> ALEEAPWPPPEGAFVGFVLSRKEPMWADLLALAAARGGRVHRAPEPYKALRDLKEARGLLAKDLSVLALREGLGLPPGDDPMLLAYLLDPSNTTPEGVARRYGGEWTEEAGERAALSERLFANLWGRLEGEERLLWLYREVERPLSAVLAHMEATGVRLDVAYLRALSLEVAEEIARLEAEVFRLAGHPFNLNSRDQ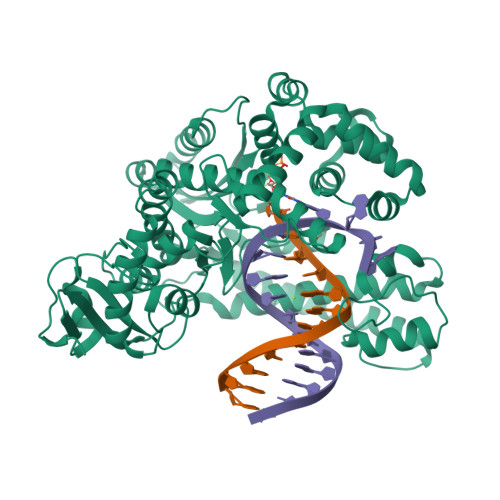LERVLFDELGLPAIGKTEKTGKRSTSAAVLEALREAHPIVEKILQYRELTKLKSTYIDPLPDLIHPRTGRLHTRFNQTATATGRLSSSDPNLQNIPVRTPLGQRIRRAFIAEEGWLLVALDYSQIELRVLAHLSGDENLIRVFQEGRDIHTETASWMFGVPREAVDPLMRRAAKTINFGVLYGMSAHRLSQELAIPYEEAQAFIERYFQSFPKVRAWIEKTLEEGRRRGYVETLFGRRRYVPDLEARVKSVREAAERKAFNMPVQGTAADLMKLAMVKLFPRLEEMGARMLLQVHDELVLEAPKERAEAVARLAKEVMEGVYPLAVPLEVEVGIGEDWLSAKE> NALPTWWKQAVFYQVYPRSFKDTNGDGIGDLNGIIENLDYLKKLGIDAIWINPHYDSPNTDNGYDIRDYRKIMKEYGTMEDFDRLISEMKKRNMRLMIDIVINHTSDQHAWFVQSKSGKNNPYRDYYFWRDGKDGHAPNNYPSFFGGSAWEKDDKSGQYYLHYFAKQQPDLNWDNPKVRQDLYDMLRFWLDKGVSGLRFATVATYSKIPNFPDLSQQQLKNFAEEYTKGPKIHDYVNEMNREVLSHYDIATAGEIFGVPLDKSIKFFDRRRNELNIAFTFDLIRLDRDADERWRRKDWTLSQFRKIVDKVDQTAGEYGWNAFFLDNHDNPRAVSHFGDDRPQWREHAAKALATLTLTQRATPFIYQGSELGMTNYPFKKIDDFDDVEVKGFWQDYVETGKVKAEEFLQNVRQTSRDNSRTPFQWDASKNAGFTSGTPWLKINPNYKEINSADQINNPNSVFNYYRKLINIRHDIPALTYGSYIDLDPDNNSVYAYTRTLGAEKYLVVINFKEEVMHYTLPGDLSINKVITENNSHTIVNKNDRQLRLEPWQSGIYKLNP

SIases, classified as glycoside hydrolase family 13 (GH13) enzymes, catalyze the isomerization of sucrose to produce isomaltulose and trehalulose as primary products and D-glucose and D-fructose as by-products. NX-5 (named NX-5 in this work) that predominantly produces isomaltulose (~87%). Similar to other GH13 family enzymes, the NX-5 molecule is composed of three domains: the N-domain (residues 42-145 and 216-520), the sub-domain (residues 146-215), and the C-domain (residues 521-600). Among them, residues Asp102, His145, Arg239, His368, Asp369, Glu428, and Arg456 are responsible for sucrose binding and residues Asp241 (the nucleophile) and Glu295 (the acid catalyst) are crucial for sucrose hydrolysis for PalI, MutB, and SmuA.

Inspired by the work from Ravaud et al., we obtained the crystals of the D241A/glucose complex by co-crystallizing the D241A mutant with sucrose. Asp241 is the key nucleophile residue involved in the catalysis of the glycosidic bond cleavage. In the 2.00 Å structure, clear electron density of D-glucose rather than sucrose was identified in the active site. This demonstrated that replacement of Asp241 with an alanine residue did not totally disrupt the hydrolytic activity of NX-5, as observed in the complex structure of MutB D200A-glucose. Moreover, the D241A/glucose complex structure may represent NX-5 in an intermediate state of the sucrose isomerization process and could be used for molecular dynamics (MD) calculations. The structures of the D241A/glucose and E295Q/sucrose complexes are highly similar with a RMSD value of 0.14 Å, indicating that little conformational change happens after sucrose hydrolysis. After sucrose hydrolysis and the exiting of fructose, their side chains bounced back to the original position in the active site pocket. To elucidate the mechanism of the product specificity of NX-5, we used the GOLD program (version 5.1, released by the Cambridge Crystallographic Data Centre) to dock fructofuranose or fructopyranose, a transition state analogue of isomaltulose or trehalulose into the active site of the D241A/glucose complex structure.> MSGQFTGTGTGGDVFKVDLNEQFDRADMVWIGTASVLVWIMIPGVGLLYSGISRKKHALSLMWAALMAACVAAFQWFWW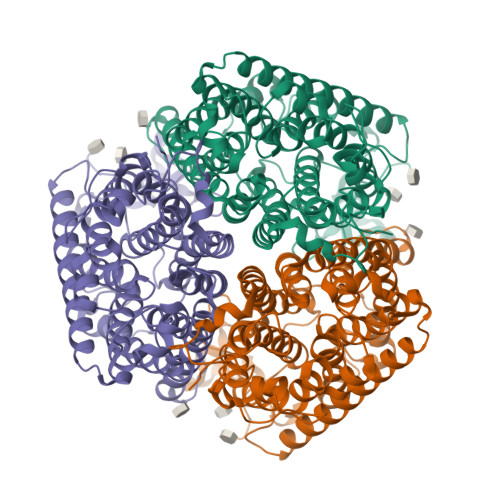GYSLVFAHNGSVFLGTLQNFCLKDVLGAPSIVKTVPDILFCLYQGMFAAVTAILMAGAGCERARLGPMMVFLFIWLTVVYCPIAYWTWGGNGWLVSLGALDFAGGGPVHENSGFAALAYSLWLGKRHDPVAKGKVPKYKPHSVSSIVMGTIFLWFGWYGFNGGSTGNSSMRSWYACVNTNLAAATGGLTWMLVDWFRTGGKWSTVGLCMGAIAGLVGITPAAGYVPVYTSVIFGIVPAIICNFAVDLKDLLQIDDGMDVWALHGVGGFVGNFMTGLFAADYVAMIDGTEIDGGWMNHHWKQLGYQLAGSCAVAAWSFTVTSIILLAMDRIPFLRIRLHEDEEMLGTDLAQIGEYAYYADDDPETNPYVLEPIRSTTISQPLPHIDGVADGSSNNDSGEAKNHHHHHH> PIVRVAVLAAGDDGGRLTEMALPSELPLREILPAVQRIVQPARENDGAADPAAAPNPVRLSLAPIGGAPFSLDATLDTVG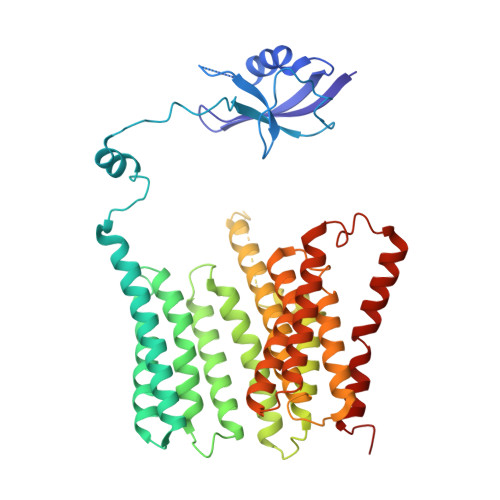VVDGDLLALQAVPSGPPAPRIVEDIADAAVIFSEARRRQWGPTHIARGAALALIGLILVGTGLSVAHRVITGDLLGQFIVSGIALATVIAALAVRNRSAVLATSLAVTALVPVAAAFALGVPGDFGAPNVLLAAAGVAAWSLISMAGSPDDRGIAVFTATAVTGVGVLLVAGAASLWVISSDVIGCALVLLGLIVTVQAAQLSAMWARFPLPVIPAPGDPTPAARPLSVLADLPRRVRVSQAHQTGVIAAGVLLGVAGSVALVSSANASPWAWYIVVAAAAGAALRARVWDSAACKAWLLGHSYLLAVALLVAFVIGDRYQAALWALAALAVLVLVWIVAALNPKIASPDTYSLPMRRMVGFLATGLDASLIPVMALLVGLFSLV>NEQLAKQKGCMACHDLKAGGGKKVGPAYADVAKKYAGRKDAVD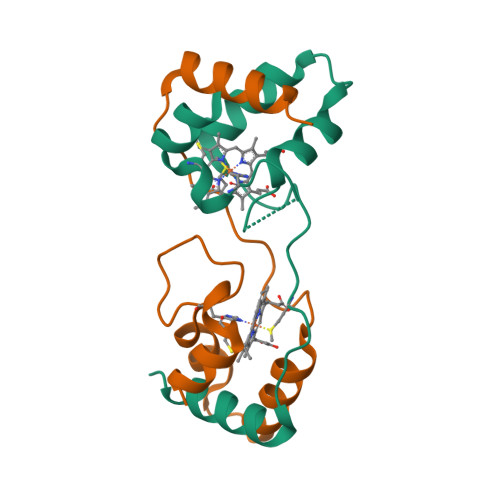YLAGKIKKGGSGVWGSVPMPPQNVTDAEAKQLAQWILSIK[2x]>[10x]MDPIRSFCGKLRSLASTLDCETARLQRALDGEESDFEDYPMRILY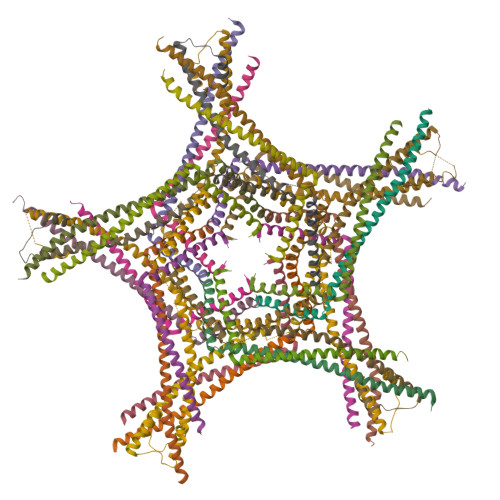DLHSEVQTLKDDINILLDKARLENQEGIDFIKATKVLMEKNSMDIMKIREYFQKYG;>[10x]MASSDLEQLCSHVNEKIGNIKKTLSLRNCGQEPTLKTVLNKIGDEIIVINELLNKLELEIQYQEQTNNSLKELCESLEEDYKDIEHLKENV;>GHMEAEVDKLELMFQKAESDLDYIQYRLEYEIKTNHPDSASEKNPVTLLKELSVIKSRYQTLYARFKPVAVEQKESKSRICATVKKTMNMIQKLQKQTDLELSPLTKEEKTAAEQFKFHMPDL[10x]> MAGGEAGVTLGQPHLSRQDLTTLDVTKLTPLSHEVISRQATINIGTIGHVAHGKSTVVKAISGVHTVRFKNELERNITIKLGYANAKIYKLDDPSCPRPECYRSCGSSTPDEFPTDIPGTKGNFKLVRHVSFVDCPGHDILMATMLNGAAVMDAALLLIAGNESCPQPQTSEHLAAIEIMKLKHILILQNKIDLVKESQAKEQYEQ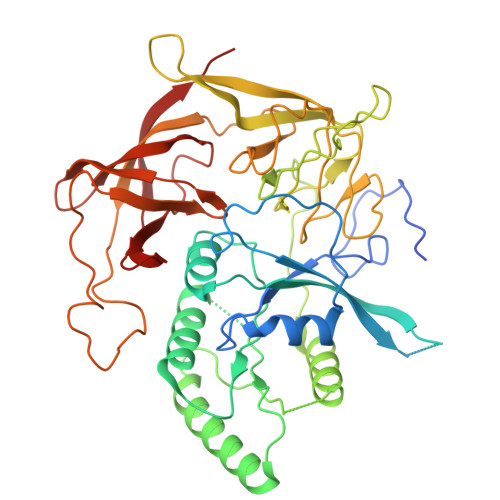ILAFVQGTVAEGAPIIPISAQLKYNIEVVCEYIVKKIPVPPRDFTSEPRLIVIRSFDVNKPGCEVDDLKGGVAGGSILKGVLKVGQEIEVRPGIVSKDSEGKLMCKPIFSKIVSLFAEHNDLQYAAPGGLIGVGTKIDPTLCRADRMVGQVLGAVGALPEIFTELEISYFLLRRLLGVRTEGDKKAAKVQKLSKNEVLMVNIGSLSTGGRVSAVKADLGKIVLTNPVCTEVGEKIALSRRVEKHWRLIGWGQIRRGVTIKPTVDDD>TGGTHTPKLKHLDKLLAHCHRRRYTAKSTIIYAGDRCETLFFIIKGSVTILIEDDDGREMIIGYLNSGDFFGELGLFEKEGSEQERSAWVRAKVECEVAEISYAKFRELSQQDSEILYTLGSQMADRLRKTTRKVGDLAFLDVTGRVARTLLDLCQQPDAMTHPDGMQIKITRQEIGRIVGCSREMVGRV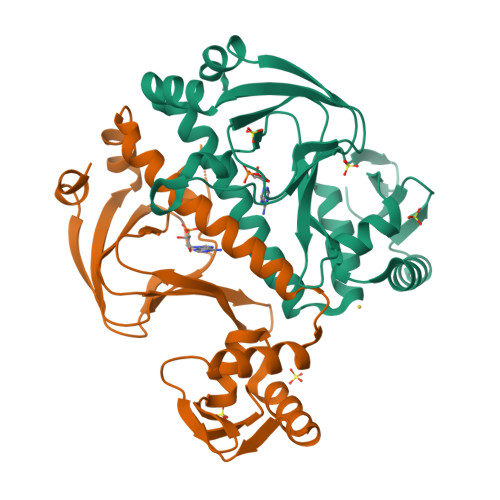LKSLEEQGLVHVKGKTMVVFGTR[2x]>GICKSSDCIKSAARLIQNMDATAEPCTDFFKYACGGWLKRNVIPETSSRYSNFDILRDELEVILKDVLQEPKTEDIVAVQKAKTLYRSCVNETAIDSRGGQPLLKLLPDVYGWPVATQNWEQTYGTSWSAEKSIAQLNSKYGKKVLINFFVGTDDKNSMNHIIHIDQPRLGLPSRDYYECTGIYKEACTAYVDFMIAVAKLIRQEEGLPIDENQISVEMNKVMELEKEIANATTKSEDRNDPMLLYNKMTLAQIQNNFSLEINGKPFSWSNFTNEIMSTVNINIPNEEDVVVYAPEYLIKLKPILTKYSPRDLQNLMSWRFIMDLVSSLSRTYKDSRNAFRKALYGTTSESATWRRCANYVNGNMENAVGRLYVEAAFAGESKHVVEDLIAQIREVFIQTLDDLTWMDAETKKKAEEKALAIKERIGYPDDIVSNDNKLNNEYLELNYKEDEYFENIIQNLKFSQSKQLKKLREKVDKDEWITGAAIVNAFYSSGRNQIVFPAGILQPPFFSAQQSNSLNYGGIGMVIGHEITHGFDDNGRNFNKDGDLVDWWTQQSANNFKEQSQCMVYQYGNFSWDLAGGQHLNGINTLGENIADNGGIGQAYRAYQNYVKKNGEEKLLPGIDLNHKQLFFLNFAQVWCGTYRPEYAVNSIKTDVHSPGNFRIIGSLQNSVE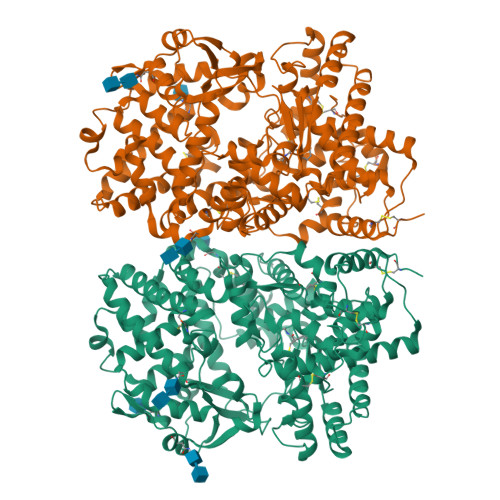FSEAFQCPKNSYMNPEKKCRVW[2x]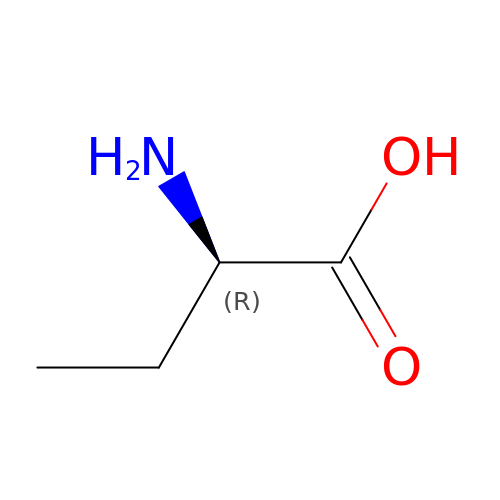D-ALPHA-AMINOBUTYRIC ACID | C4 H9 N O2 | QWCKQJZIFLGMSD-GSVOUGTGSA-N> APADKPQVLASFTQTSASSQNAWLAANRNQSAWAAYEFDWSTDLCTQAPDNPFGFPFNTACARHDFGYRNY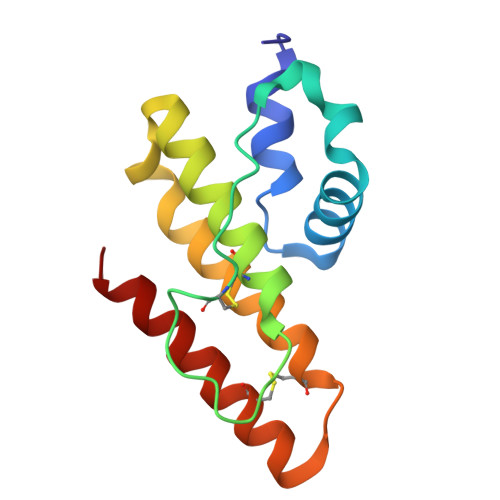KAAGSFDANKSRIDSAFYEDMKRVCTGYTGEKNTACNSTAWTYYQAVKIFG>[4x]MVTAHFVLIHTICHGAWIWHKLKPALERAGHKVTALDMAASGIDPRQIEQINSFDEYSEPLLTFLEKLPQGEKVIIVGESCAGLNIAIAADRYVDKIAAGVFHNSLLPDTVHSPSYTVEKLLESFPDWRDTEYFTFTNITGETITTM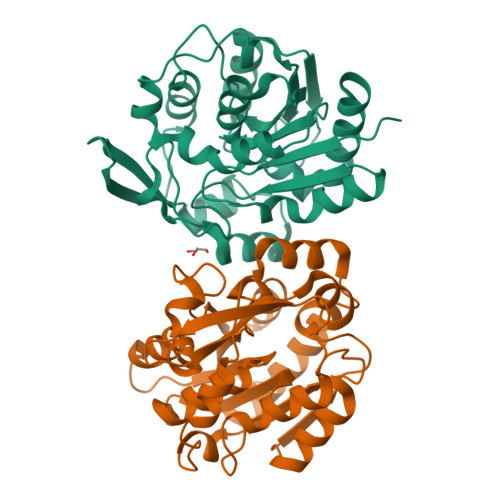KLGFVLLRENLFTKCTDGEYELAKMVMRPGSLFQNVLAQRPKFTEKGYGSIKKVYIWTDQDKIFLPDFQRWQIANYKPDKVYQVQGGDHKLQLTKTEEVAHILQEVADAYA7-methyl-2-morpholin-4-yl-9-[(1~{R})-1-phenylazanylethyl]-3~{H}-pyrido[1,2-a]pyrimidin-4-one 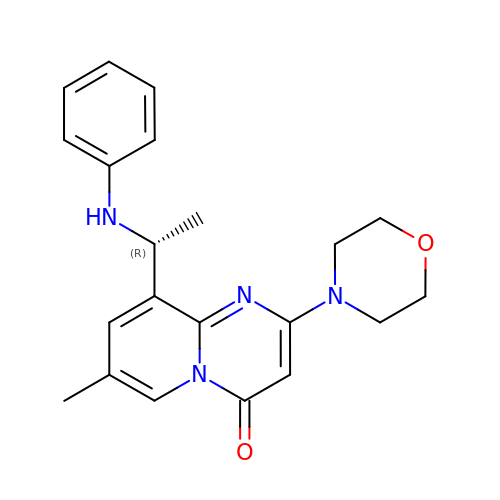| C21 H24 N4 O2 | CPRAGQJXBLMUEL-MRXNPFEDSA-N> GSHMPAGGDPIKSLLVVGGARSGKSRFAQRMAEASGRSLVLIATAQPLDAEMADRISRHAADRDARWTLIEAFFDLGQTLRREAQPERLLVVDSVTLWLSNLLLRGDDLSPPIKDLARTAARLEGPVIFVSNEVGAGIVPDNAL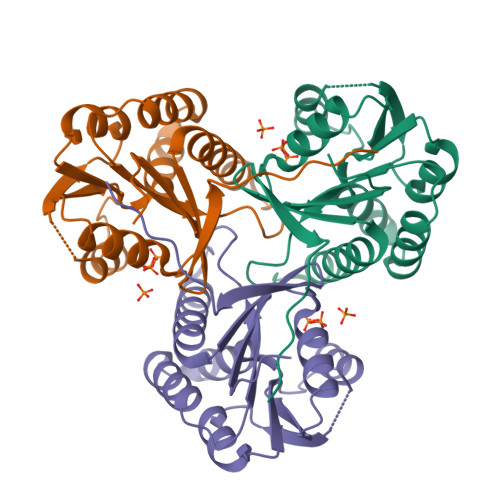ARAFRDAQGMCNQRLAEACDAVTLVTAGIATQIKPGPEPVFRF>[2x]MPKTLTEKLNAIKAAGKGIFVPYIMAGDHEKGLDGLAETIHFLEDLGVSAIEVGIPFSDPVADGPVIEEAGLRSLAHGTSTQALVETLKTIETEIPLVIMTYFNPLFQYGVENFVKDLADTAVKGLIIPDLPHEHANFVEPFLANTDIALIPLVSLTTGIERQKELIEGAEGFIYAVAINGVTGKSGNYRADLDKHLAQLHQVADIPVLTGFGVSSQADLERFNAVSDGVIVGSKIVKALHQGEPIQDFIRQAVAYQK;>SNAQEPNKDGFYGKFGGRFVPETLMTAVLELEKAYRESQADPSFQEELNQLLRQYVGRETPLYYAKNLTQHIGGAKIYLKREDLNHTGAHKINNALGQVWLAKRMGKKKIIAETGAGQHGVATATAAALFNMECTIYMGEEDVKRQALNVFRMELLGAKVEAVTDGSRVLKDAVNAALRSWVANIDDTHYILGSALGPHPFPEIVRDFQSVIGREAKQQYRDLTGRDLPDALVACVGGGSNAIGLFHPFVEDESVAMYGTEAAGLGVDTEHHAATLTKGRPGVLHGSLMDVLQDAHGQILEAFSISAGLDYPGIGPEHSHYHDIKRASYVPVTDEEALEGFQLLSRVEGIIPALESSHAIAFAVKLAKELGPEKSMIVCLSGRGDKDVVQVKDRLEADAAKKGEAHA[2x]

Tryptophan synthase (TrpAB) is a pyridoxal 5′-phosphate (PLP)-dependent enzyme that participates in the final two steps of tryptophan synthesis in plants, fungi and bacteria. The enzyme consists of two protein chains, α (TrpA) and β (TrpB), that operate as a linear αββα heterotetrameric complex containing two functional TrpAB units. In bacteria, TrpA and TrpB are encoded by usually adjacent trpA and trpB genes that belong to the highly regulated tryptophan-biosynthesis operon. The TrpA subunit converts indole-3-glycerol phosphate (IGP) into glyceraldehyde 3-phosphate (G3P) and indole (IND).

The structure, which was determined at 2.45 Å resolution, was solved by molecular replacement. In chains A and C, corresponding to TrpA (amino-acid residues 1–258), residues 1, 180–189 and 182–187, respectively, were not modeled owing to a lack of interpretable electron density. The structures of the FtTrpAB and SpTrpAB αββα heterotetramers provide a new set of high-quality models and enable comparison of the intermolecular tunnel connecting the TrpA and TrpB catalytic pockets. In contrast to the active sites, the composition of the tunnel, which is mostly encompassed by TrpB, varies between the orthologs, although generally SpTrpAB shares some features with MtTrpAB while FtTrpAB is similar to StTrpAB. For example, one side of the SpTrpB tunnel contains βTyr311, βHis285 and the neighboring βLeu284, with the tyrosine rotated towards the active site of TrpB, where it could potentially interfere with the β reaction. The opposite side contributes βVal174, βLeu178 and βLeu192. While no monovalent cations have been modeled in the current structures, by analogy to the data collected from the MtTrpAB and StTrpAB systems the MVC must be created by βTyr311Sp, βGly313Sp, βAla273Sp, βGly237Sp and βThr275Sp in SpTrpAB and βPhe305Ft, βSer307Ft, βGly267Ft, βGly231Ft in FtTrpAB, with βPro269Ft replacing the threonine residue. In the SpTrpAB βeO state there is also a hydrogen bond between the αSer58 carbonyl group and βLys171, but βArg179 is too distant to interact with the catalytic aspartate. The activation of SpTrpAB by the α-binders is unexpected and surprising. The weak inhibition of SpTrpAB, which carries the smallest side chain among the tested enzymes (αVal61 in place of αGly66 in MtTrpAB, αLeu59 in FtTrpAB and αMet58 in LpPhTrpAB), supports the previous conclusion that any substitution in the loop would drastically reduce the size of the BRD4592 binding pocket, limiting the inhibitor affinity.> GIDPFTDDLEQYLDEKILRLKDEMNIAAQLDIDTLNKRIETGDTSLIAMQKVKLLPKVVSVLSKANLADTILDNNLLQSVRIW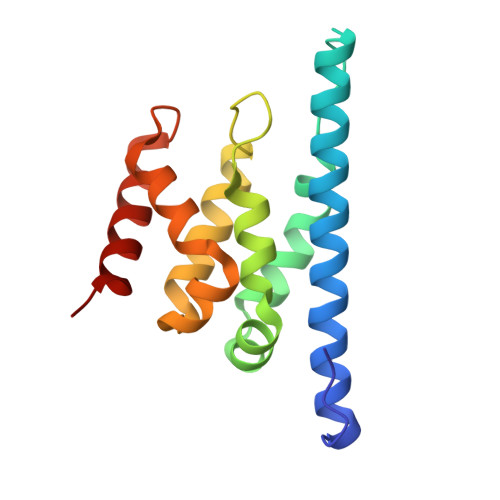LEPLPDGSLPSFEIQKSLFAALNDLPVKTEHLKESGLGRVVIFYTKSKRVEAQLARLAEKLIAEWTRP>MSLSEIKRKFDAVSGKYDEQRRKFIPCFDDFYGVSVSIASVDTENPDILDLGAGTGLLSAFLMEKYPEATFTLVDMSEKMLEIAKNRFRGNLKVKYIEADYSKYDFEEKYDMVVSALSIHHLEDEDKKELYKRSYSILKESGIFINADLVHGETAFIENLNKTIWR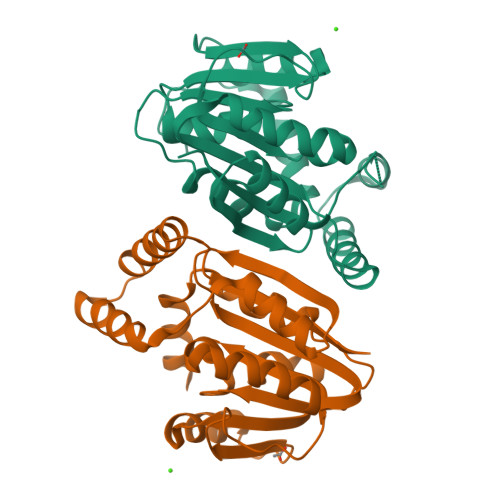QYVENSGLTEEEIAAGYERSKLDKDIEMNQQLNWLKEAGFRDVSCIYKYYQFAVMFGRKTEGHHHHHH[2x]> MARENEMDENLEQVSGIIGNLRHMALDMGNEIDTQNRQIDRIMEKADSNKT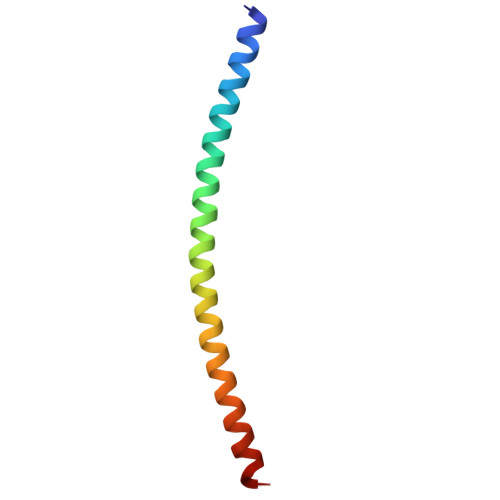RIDEANQRATKMLG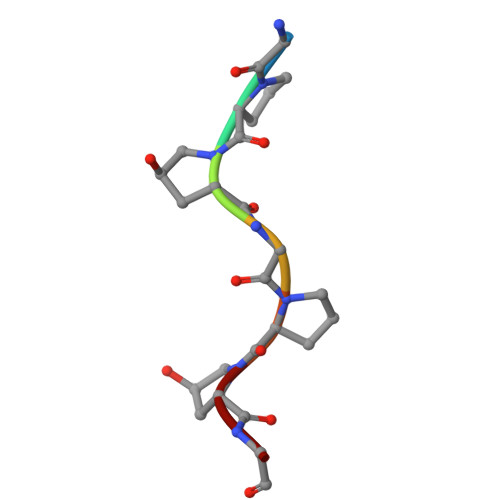> GPPGPPG[(2E)-1-{4-[(2-chlorophenyl)amino]-4-oxobutanoyl}-2-(naphthalen-1-ylmethylidene)hydrazino]acetic 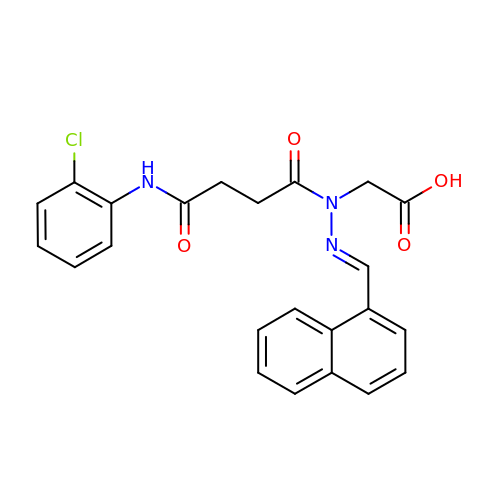acid | C23 H20 Cl N3 O4 | HHHUDHYQFQBYIZ-AFUMVMLFSA-N>ITGQAACPESWIGFQRKCFYFSDDTKNWTSSQRFCDSQDADLAQVESFQELNFLLRYKGPSDHWIGLSREQGQPWKWINGTEWTRQFPI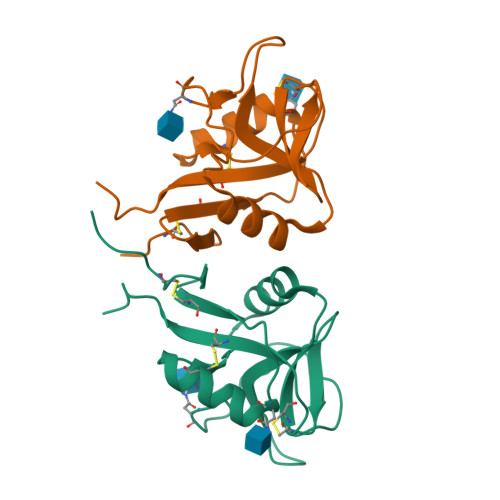LGAGECAYLNDKGASSARCYTERKWICSKSDIHVGTKHHHHHHHHG[2x]> VPEITTAQTIANSVVDAKKFDYLFGKATGNSHTLDRTNQLALEMKRLGVADDINGHAVLAEHFTQATKDSNNIV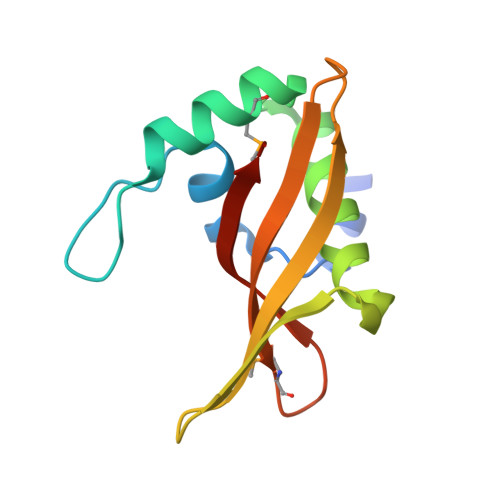KKYTDQYGSFEIRESFFIGPSGKATVFESTFEVMKDGSHRFITTIPKNGVTK>MAHHHHHHMDIRYFGTTPRYSEAVGANGLIFLSGMVPENGETAAEQTADVLA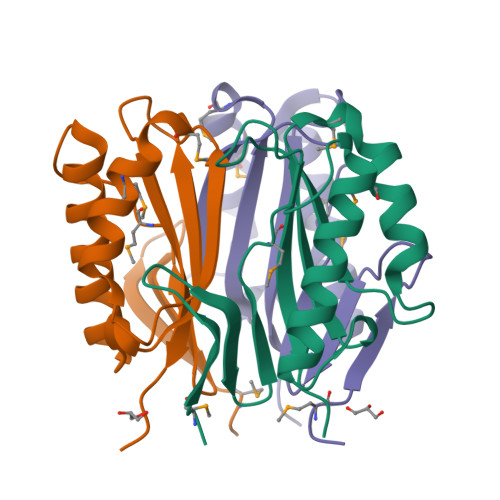QIDRWLAECGSDKAHVLDAVIYLRDMGDYAEMNGVWDAWVAAGRTPARACVEARLARPEWRVEIKITAVKRDAATA[12x]> ALSYSSPLRFFRNFRFHPEFTRLVAGGWRSLTYSSRIDPDKEMCPYELEGTQCPSGCSFQHFVDITPA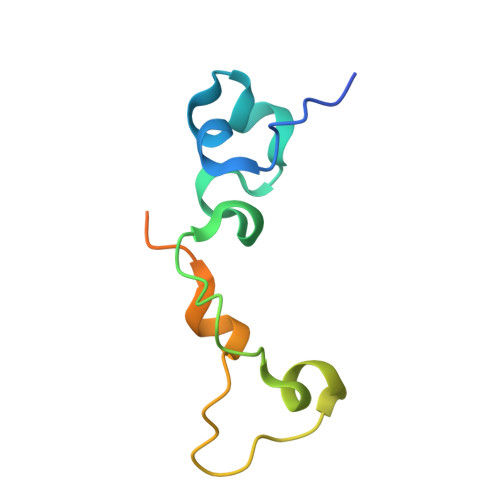ADERILLELSGSHHHHHH2-phenylpyridin-4-amine | C11 H10 N2 | 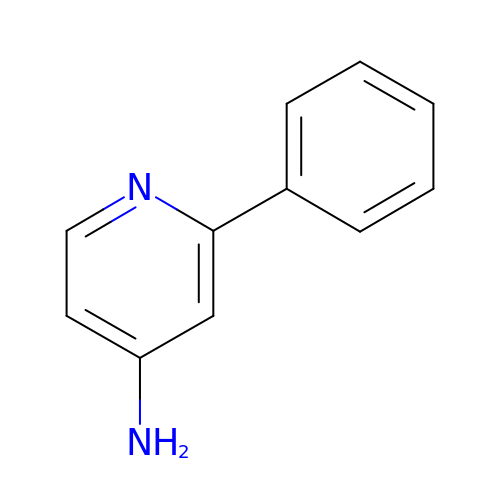CHVKPWIABFICLK-UHFFFAOYSA-N> WVIPPISCPENEKGEFPKNLVQIKSNRDKETKVFYSITGQGADKPPVGVFIIERETGWLKVTQPLDREAIAKYILYSHAVSSNGEAVEDPMEIVITVTDQNDNRPEFTQEVFEGSVAEGAVPGTSVMKVSATDADDDVNTYNAAIAYTIVSQDPELPHKNMFT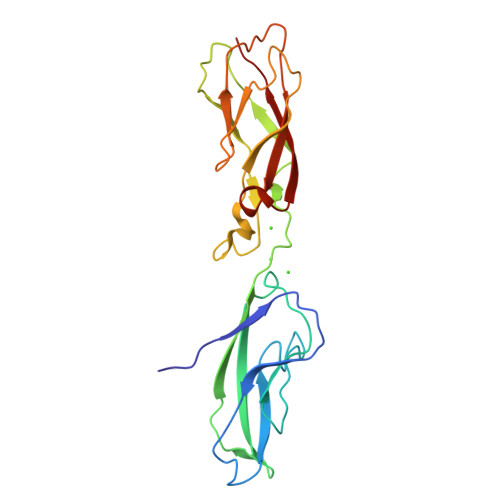VNRDTGVISVLTSGLDRESYPTYTLVVQAADLQGEGLSTTAKAVITVKD>MLRRLPTSCFLKRSQFRGFAATSPLLNLDYQMYRTATVREAAPQFSGQAVVNGAIKDINMNDYKGKYIVLFFYPMDFTFVCPTEIIAFSDRHADFEKLNTQVVAVSCDSVYSHLAWVNTPRKKGGLGEMHIPVLADKSMEIARDYGVLIEESGIALRGLFIIDKK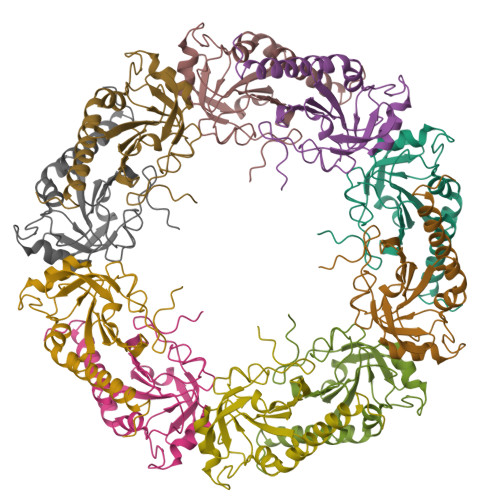GILRHSTINDLPVGRNVDEALRVLEAFQYADENGDAIPCGWKPGQPTLDTTKAGEFFEKNM[10x]>[12x]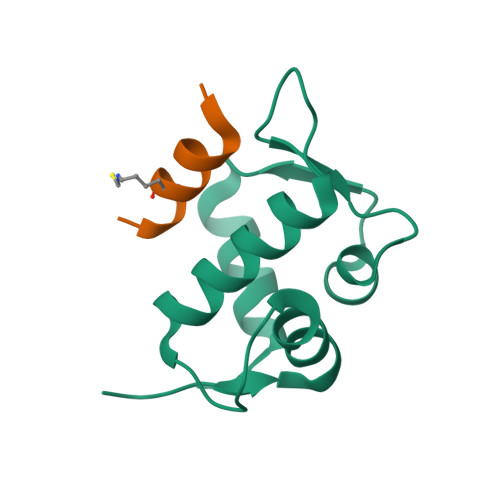ETLVRPKPLLLKLLKSVGAQKDTYTMKEVLFYLGQYIMTKRLYDEKQQHIVYCSNDLLGDLFGVPSFSVKEHRKIYTMIYRNLVV;>[12x]XTSFAEYWKLLSCX>GAMVMRLGDAAELCYNLTSSYLQIAAESDSIIAQTQRAINTTKSILINETFPKWSPLNGEISFSYNGGKDCQVLLLLYLSCLWEYYIVKLSQSQFDGKFHRFPLTKLPTVFIDHDDTFKTLENFIEETSLRYSLSLYESDRDKCETMAEAFETFLQVFPETKAIVIGIRHTDPFGEHLKPIQKTDANWPDFYRLQPLLHWNLANIWSFLLYSNEPICELYRYGFTSLGNVEETLPNPHLRKDKNSTPLKLNFEWEIENRYKHNEVTKAEPIPIADE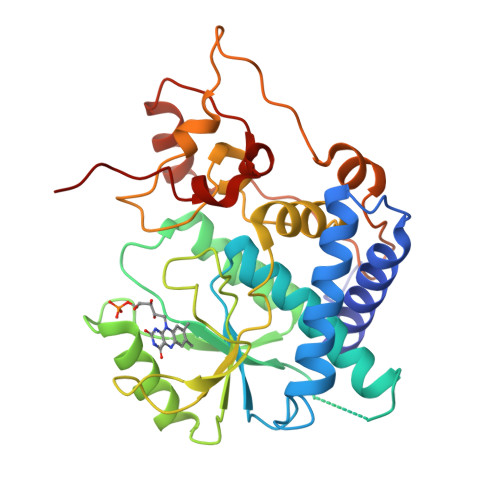DLVKIENLHEDYYPGWYLVDDKLERAGRIKKK[6x]>[2x]MQQVRQS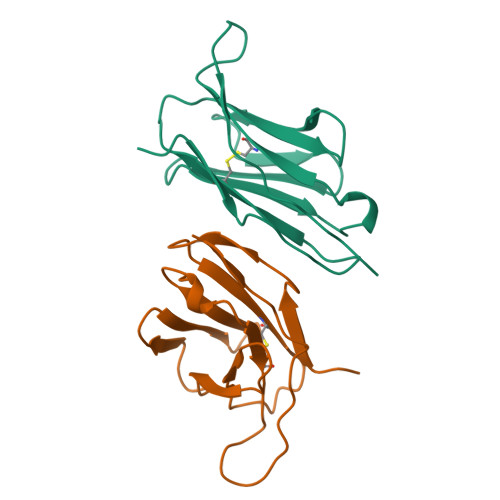PQSLTVWEGETAILNCSYENSAFDYFPWYQQFPGEGPALLISILSVSNKKEDGRFTIFFNKREKKLSLHIADSQPGDSATYFCAASASFGDNSKLIWGLGTSLVVNP> SA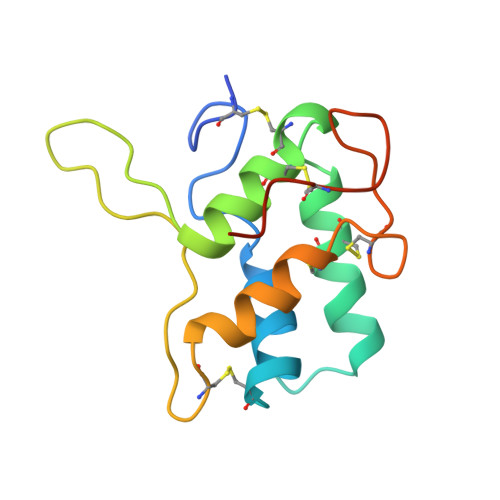GTSCVPGWAIPHNPLPSCRWYVTSRTCGIGPRLPWPELKRRCCRELADIPAYCRCTALSILMDGAIPPGPDAQLEGRLEDLPGCPREVQRGFAATLVTEAECNLATISGVAECPWILGGGTMPSK> MIWMFAAAAAQMIQGGLQYAQDAKNQRRQNKADQKYNEAVRSASARQITEINTQRSVSRAQTAQALDAARRQGAGESSARNLQAAATDTMGASVEQNLQEVGVQLAAAEGNLMQNAELTELSLDSSVMNTVDQARNSIRELSNPLGTDWAATGSAVGQIGTSMVANKLGGQGWFGGNSGTQQPAPI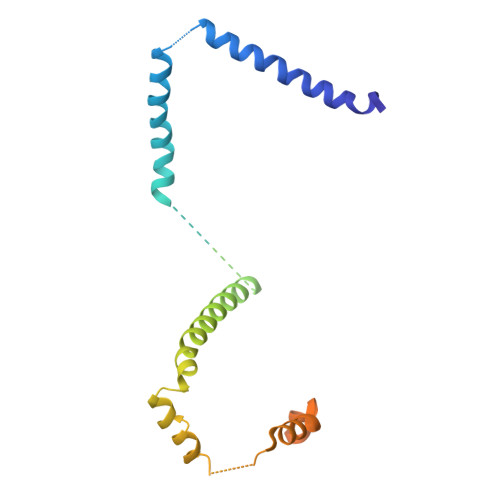SQAAPPTRSNNLSTRLNV>MIVLFVDFDYFYAQVEEVLNPSLKGKPVVVCVFSGRFEDSGAVATANYEARKFGVKAGIPIVEAKKILPNAVYLPMRKEVYQQVSSRIMNLLREYSEKIEIASIDEAYLDISDKVRDYREAYNLGLEIKNKILEKEKITVTVGISKNKVFAKIAADMAKPNGIKVIDDEEVKRLIRELDIADVPGIGNITAEKLKKLGINKLVDTLSIEFDKLKGMIGEAKAKYLISLARDEYNEPIRTRVRKSIGRYLTL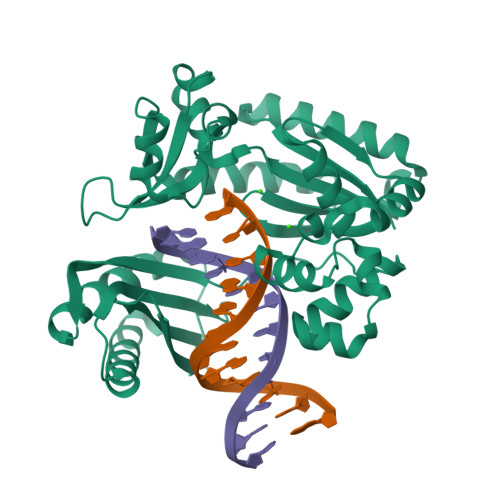PYNTRDVKVILPYLKKAINEAYNKVNGIPMRITVIAIMEDLDILSKGKKFKHGISIDNAYKVAEDLLRELLVRDKRRNVRRIGVKLDNIIINKTNLSDFFDIGGHHHHHH[2x]> GWELQAQNPHERGPDPSNSYIEQARGSYSVSQRSISRLGSDGFRDGTMYYPTSTADGRFGVVAISPGYTASESTIAWLGPRLASFGFVVVTINTDSRYDQPRQRATQLHAALDHAIGDSVVGPRIDTSRQAVMGHSMGGGGALQAAEERDEIRAAVPLTPWNLKKGWSGVDAATLVIGAENDAIAPVRSHSIPFYESLTNAERRAYLELRREGHFAPNSSNTLIAKYSVSWLKRYVDNDLRYDQFIDPGPR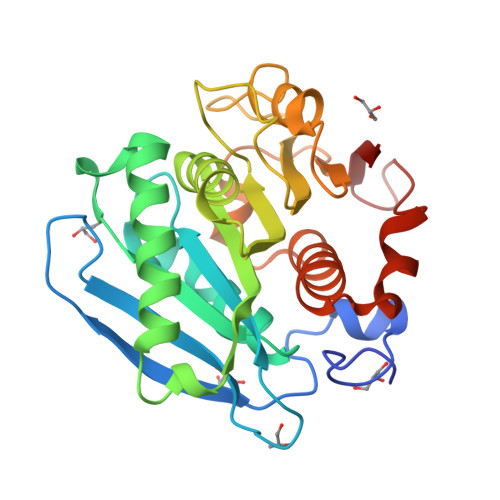TGITTGVSDYRLG>MEAEQRPAAGASEGATPGLEA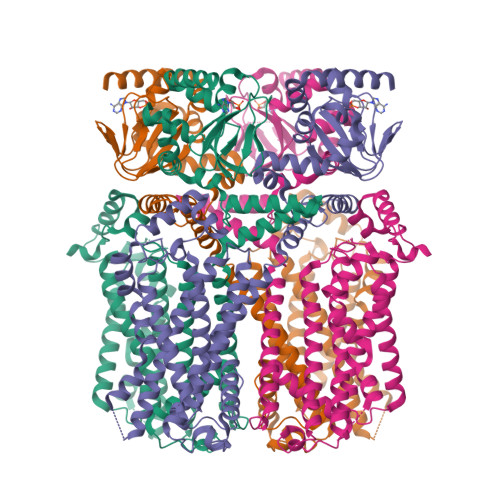VPPVAPPPATAASGPIPKSGPEPKRRHLGTLLQPTVNKFSLRVFGSHKAVEIEQERVKSAGAWIIHPYSDFRFYWDLIMLLLMVGNLIVLPVGITFFKEENSPPWIVFNVLSDTFFLLDLVLNFRTGIVVEEGAEILLAPRAIRTRYLRTWFLVDLISSIPVDYIFLVVELEPRLDAEVYKTARALRIVRFTKILSLLRLLRLSRLIRYIHQWEEIFHMTYDLASAVVRIFNLIGMMLLLCHWDGCLQFLVPMLQDFPPDCWVSINHMVNHSWGRQYSHALFKAMSHMLCIGYGQQAPVGMPDVWLTMLSMIVGATCYAMFIGHATALIQSLDSSRRQYQEKYKQVEQYMSFHKLPADTRQRIHEYYEHRYQGKMFDEESILGELSEPLREEIINFTCRGLVAHMPLFAHADPSFVTAVLTKLRFEVFQPGDLVVREGSVGRKMYFIQHGLLSVLARGARDTRLTDGSYFGEICLLTRGRRTASVRADTYCRLYSLSVDHFNAVLEEFPMMRRAFETVAMDRLLRIGKKNSILQRKRSEPSPGSSGGIMEQHLVQHDRDMARGVRGRAPSTGAQLSGKPVLWEPLVHAPLQAAAVTSNVAIALTHQRGPLPLSPDSPATLLARSAWRSAGSPASPLVPVRAGPWASTSRLPAPPARTLHASLSRAGRSQVSLLGPPPGGGGRRLGPRGRPLSASQPSLPQRATGDGSPGRKGSGSERLPPSGLLAKPPRTAQPPRPPVPEPATPRGLQLSANM[4x]> MSMTEFTLLRWLREGRQSRKLILLIVFIALLLDNMLLTVVVPIIPSYLYSMTHESNNTHDGSIPPAAPSGFHSIFSYYDNTTVITTNFTSSDQLQQSALTPTTSPSLATPPASADCPKADSSLLNENVKVGLLFASKATVQLLTNPFIGPMTNRIGYQIPMFAGFCIMFVSTIMFAFSGTYTLLFIARSLQGIGSSCSSVAGMGMLASVYTDDEERGNAMGVALGGLAMGVLVGPPFGSILYEFVGKTAPFIVLAVLVLFDGALQLFVLQPSRVQPESQTGTPLLTLIRDPYILIAAGSICFANMAIAMLEPALPIWMMETMCSRKWQLGVAFLPASISYLLGTNIFGPLAHKMGRWLCAFIGMIMVGISIICVPFARNIYGLIAPNFGVGFAIGMVDSSMMPIMGYLVDLRHVSVYGSVYAIADVAFCMGFAFGPSAGGAIAKSIGFPWLMTIIGVVDILFAPLCLFLRSPPAREEKMAILMDHKCPVKTKMYTQNSGQPYYTGEEEESESDE

Vesicular monoamine transporter 2 (VMAT2) is responsible for H+-dependent uptake of monoamine neurotransmitters, e.g. dopamine (DA) and serotonin (SER), from the cytoplasm to presynaptic vesicles in monoaminergic neurons. Vesicular monoamine transporter 2 (VMAT2) belongs to the major facilitator superfamily (MFS), and mediates cytoplasmic monoamine packaging into presynaptic vesicles. Substrates bind to MFS transporters between N-domain and C-domain, and are transported by a rocker-switch alternating access mechanism. In this work, we report two cryo-EM structures of VMAT2, with VMAT2 from Xenopus laevis adopting a canonical MFS fold and an engineered VMAT2 from Ovis aries adopting a non-canonical fold.

Eventually, the structure of XlVMAT2WT was determined at 4.0 Å resolution after extensive data collection and processing. A total of 348 out of 514 residues were traced in the XlVMAT2WT structure, including all 12 TM helices and several connecting loops. Intriguingly, comparison to the hMCT2 structure revealed that the XlVMAT2WT structure adopts a canonical MFS fold. Unlike OaVMAT2TM8/9-BRIL, N- and C-domains of XlVMAT2WT are structurally similar, and could be superimposed with a Cα RMSD of 2.5 Å. The XlVMAT2WT structure was solved in an apo, lumen-facing open conformation with a large, deep cavity. Serotonin was placed in a pocket between TM5, TM7, TM8, TM10 and TM11 near the center of XlVMAT2WT. Meanwhile, the hydroxyl group of serotonin forms a hydrogen bond with the side chain of E311 (TM7), and its amine group interacts with side chains of N304 (TM7) and D398 (TM10) via a hydrogen bond and a salt bridge, respectively. Meanwhile, purified XlVMAT2WT showed reasonable binding affinities for substrates dopamine (Kd = 1.13 ± 0.52 μM) and serotonin (Kd = 0.43 ± 0.22 μM), and for the inhibitor reserpine (Kd = 17.0 ± 8.8 nM). The non-canonical structure of OaVMAT2TM8/9-BRIL forms a dimer, whereas the canonical structure of XlVMAT2WT is a monomer.2-METHYL-BUTYRIC ACID 3-(3-FORMYLAMINO-2-HYDROXY-BENZOYLAMINO)-8-HEPTYL-2,6-DIMETHYL-4,9-DIOXO-[1,5]DIOXONAN-7-YL 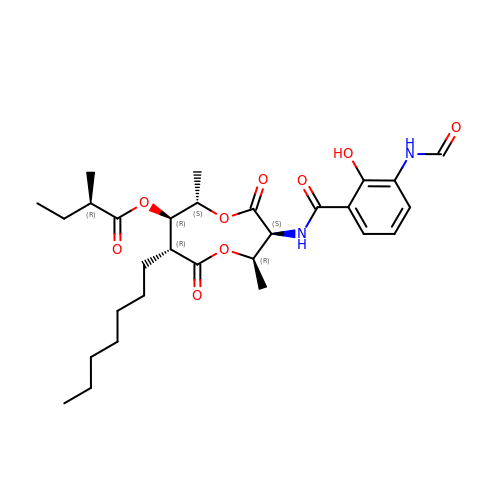ESTER | C29 H42 N2 O9 | BSSBWOQOFMLGAF-GMRPKDQWSA-N4-(6-ethoxynaphthalen-2-yl)-6-(piperazin-1-ylmethyl)-2H-indazol-3-amine 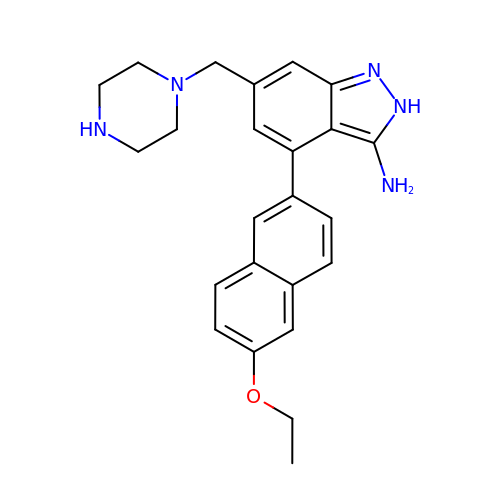| C24 H27 N5 O | ZBGMTSWSDGHDMV-UHFFFAOYSA-N> MSAVQLLWMPVVLCVMQGRLSNGACVEVDSDTEAVVGHGFKLGCISCKMRGEVQASATVDWWFMAKGESEFSHIYSYID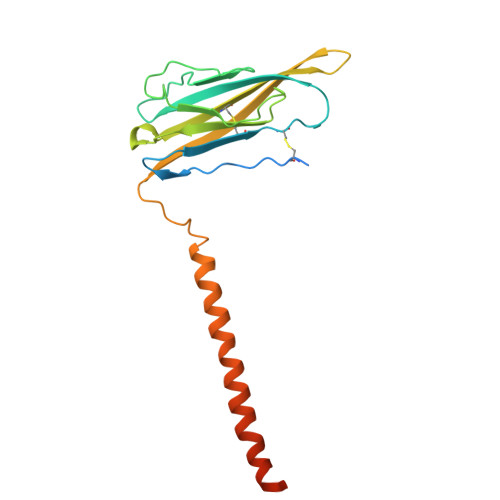MTGMVNDERFLDRLNWMGSKNTFDLQDGSIYILNVTLNDTGTYRCYFDRTLTFNYYEFRTNINKTITLNVVPKATRGTASILSEVMMYVSIIGLQLWLLVEMVYCYRKIAAAGEEALRESAAKPPLKLHP>[4x]MGSSHHHHHHSSENLYFQGHIETLPDSFTFYDGTKVQRLSDWPKRAQELKDLYQFYMYGYKPDTSVEDVTYSVNGNTLTITVKVGDKQASFNATVRLPQANSGYQPPYPVIISLGYLAGFNWQTWQFIDYSTNAVNRGYAVISFMPNDVARDDSSYTGAFYTLYPHSNKVENDTGVLMAWAWGASKILDALEKGAIPEIDAKKAIVTGF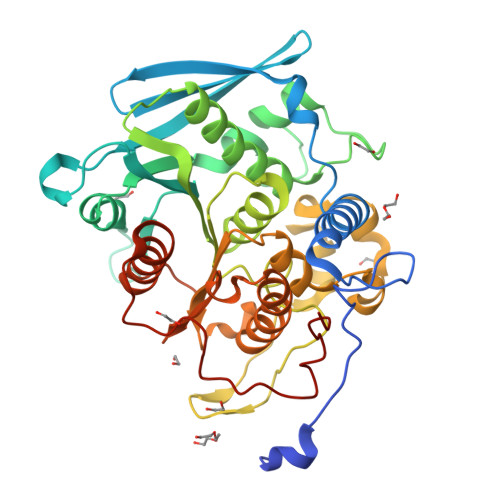SRYGKAALVAGAFDERFAVVNPHASGQGGAASFRYSFAGKQYSWGVAGNAEAFSNLQGNTEGHWFNAVFREFKDPRQLPFDQHELIALCAPRTVLITGGYSDWGTNPEGTWVSFVGARKVYEFLGVADRIGFALRDGSHAITEEDVNNLLDFCDWQLRGIQPTKDFSTSRFAIDPAWDTISVPTLYRNAD v-coelenterazine | C28 H21 N3 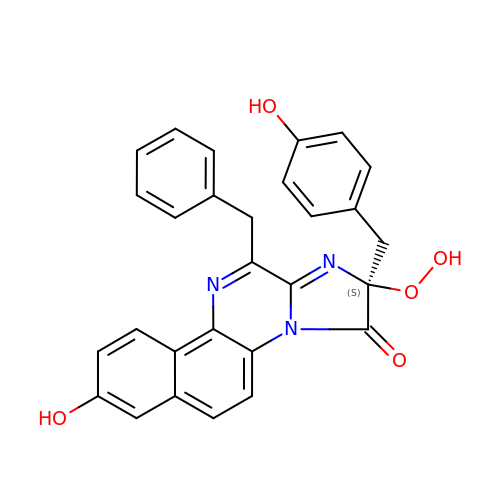O5 | ZSLLQPODRCGPLM-NDEPHWFRSA-N> LETPGQYLVYNGDLVEYEADHMAQLQRVHGFLMNDCLLVATWLPQRRGMYRYNALYPLDRLAVVNVKDNPPMKDMFKLLMFPESRIFQAENAKIKREWLEVLEETKRALSDKR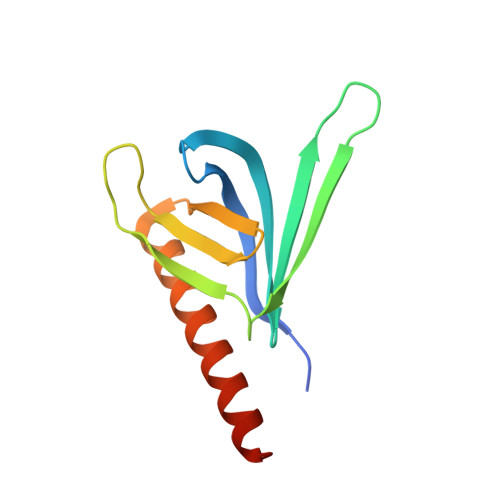RREQEEA>[2x]GAMGSMTNSVKTNGPSSSDMEYYYKSLYPFKHIFNWLNHSPKPSRDMINREFAMAFRSGAYKRYNSFNSVQDFKAQIEKANPDRFEIGAIYNKPPRERDTLLKSELKALEKELVFDIDMDDYDAFRTCCSGAQVCSKCWKFISLAMKITNTALREDFGYKDFIWVFSGRRGAHCWVSDKRARALTDVQRRNVLDYVNVIRDRNTDKRLALKRPYHPHLARSLEQLKPF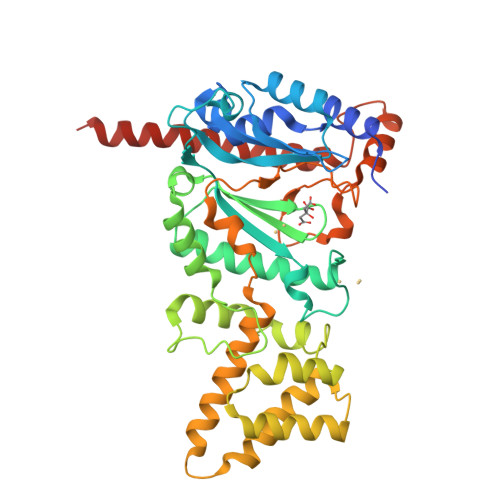FVSIMLEEQNPWEDDQHAIQTLLPALYDKQLIDSLKKYWLDNPRRSSKEKWNDIDQIATSLFKGPKQDSHIIKLRECKEDLVLMTLYPKLDVEVTKQTIHLLKAPFCIHPATGNVCVPIDESFAPEKAPKLIDLQTEMEKNNDVSLTALQPFINQFQAYVSSLLKNELGSVKREREDDDEPASLDF> MGSSHHHHHHSQDPNSMTTLTRQDLNFGQVVADVLCEFLEVAVHLILYVREVYP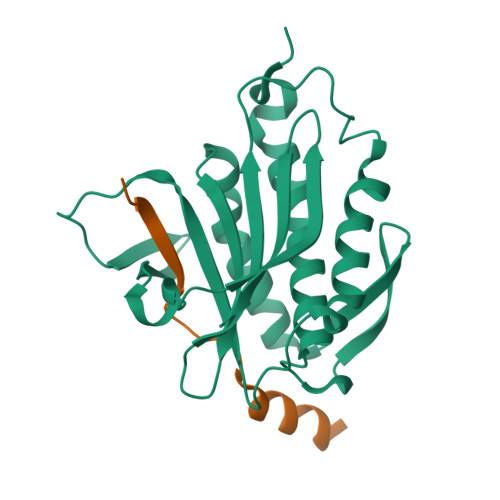VGIFQARKKYNVPVQMSCHPELNQYIQDTLHCVKPLLEKNDVEKVVVVILDKEHRPVEKFVFEITQPPLLSISSDSLLSHVEQLLAAFILKISVCDDVLDHNPPGCTFTVLVHTREAATRNMEKIQVIKDFPWILADEQDVHMHDPRLIPLKTMTSDILKMQLYVEERAHKGS;> MEDKKIVIMPCKCAPSRQLVQVWLQAKE> SPDSAKISKEQLKKLHSNILNEIFSQSQ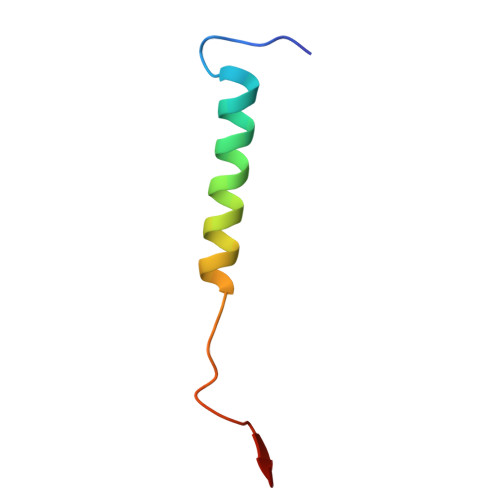VNKPGPLTVPF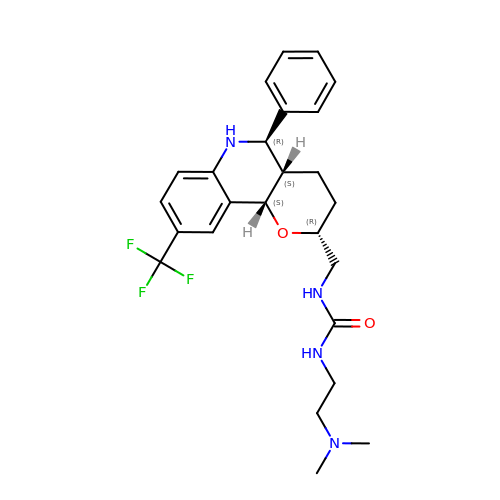1-[2-(dimethylamino)ethyl]-3-{[(2R,4aS,5R,10bS)-5-phenyl-9-(trifluoromethyl)-3,4,4a,5,6,10b-hexahydro-2H-pyrano[3,2-c]quinolin-2-yl]methyl}urea | C25 H31 F3 N4 O2 | MARIUIDCPUZLKZ-FUKQBSRTSA-N> GASPHSIESSNDWNVEKRSIRDVPVVRLPADSPIPERGDLSCRMHTCFDVYRCGFNPKNKIKVYIYALKKYVDDFGVSVSNTISREYNELLMAISDSDYYTDDINRACLFVPSIDVLNQNTLRIKETAQAMAQLSRWDRGTNHLLFNMLPGGPPDYNTALDVPRDRALLAGGGFSTWTYRQGYDVSIPVYSPLSAEVDLPEKGPGPRQYFLLSSQVGLHPEYREDLEALQVKHGESVLVLDKCTNLSEGVLSVRKRCHKHQVFDYPQVLQEATFCVVLRGARLGQAVLSDVLQAGCVPVVIADSYILPFSEVLDWKRASVVVPEEKMSDVYSILQSIPQRQIEEMQRQA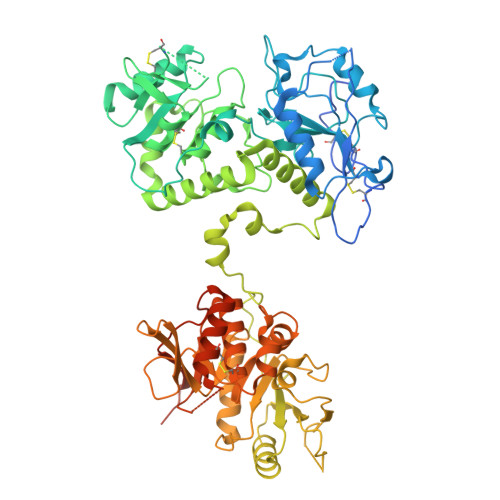RWFWEAYFQSIKAIALATLQIINDRIYPYAAISYEEWNDPPAVKWGSVSNPLFLPLIPPQSQGFTAIVLTYDRVESLFRVITEVSKVPSLSKLLVVWNNQNKNPPEDSLWPKIRVPLKVVRTAENKLSNRFFPYDEIETEAVLAIDDDIIMLTSDELQFGYEVWREFPDRLVGYPGRLHLWDHEMNKWKYESEWTNEVSMVLTGAAFYHKYFNYLYTYKMPGDIKNWVDAHMNCEDIAMNFLVANVTGKAVIKVTPRKKFKCPECTAIDGLSLDQTHMVERSECINKFASVFGTMPLKVVEHRADPVLYKDDFPEKLKSFPNIGSLNNNNNNGHHHHHHHH>GHMSYSITLRVYQTNRDRGYFSIVEKTVWHFANGGTWSEANGAHTLTMGGSGTSGMLRFMSTKGERITVAVGVHNYKRWCDVVTGLKPDETALVINPQYYNNGG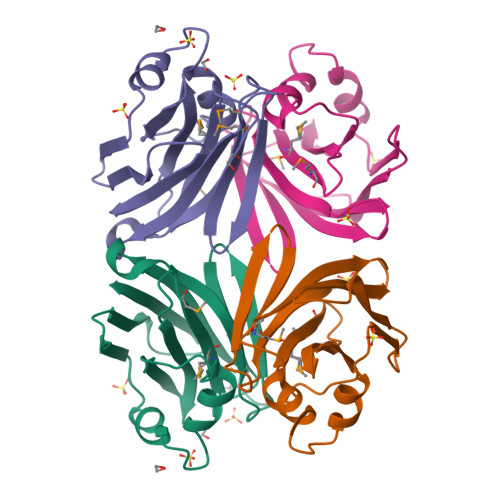RDYVREKQLAEYSVTSAIGTKVEVVYTVAEGNNLEANVIFS[2x]>[2x]TATDNARQVTIIGAGLAGTLVARLLA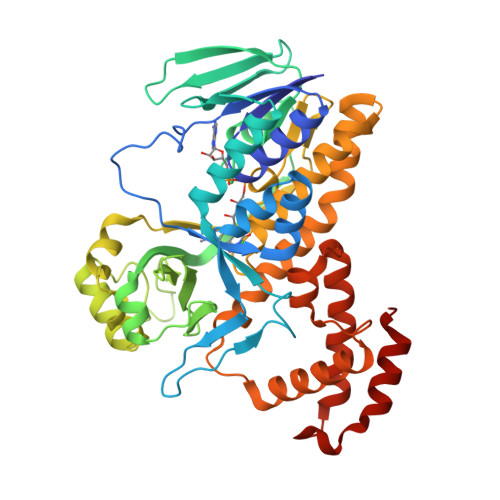RNGWQVNLFERRPDPRIETGARGRSINLALAERGAHALRLAGLEREVLAEAVMMRGRMVHVPGTPPNLQPYGRDDSEVIWSINRDRLNRILLDGAEAAGASIHFNLGLDSVDFARQRLTLSNVSGERLEKRFHLLIGADGCNSAVRQAMASVVDLGEHLETQPHGYKELQITPEASAQFNLEPNALHIWPHGDYMCIALPNLDRSFTVTLFLHHQSPAAQPASPSFAQLVDGHAARRFFQRQFPDLSPMLDSLEQDFEHHPTGKLATLRLTTWHVGGQAVLLGDAAHPMVPFHGQGMNCALEDAVALAEHLQSAADNASALAAFTAQRQPDALAIQAMALENYVEMSSKVASPTYLLERELGQIMAQRQPTRFIPRYSMVTFSRLPYAQAMARGQIQEQLLKFAVANHSDLTSINLDAVEHEVTRCLPPLSHLS Versatile peroxidase (VP, EC 1.11.1.16) constitutes the third family of ligninolytic peroxidases, which was described 20-years ago. VP combines catalytic properties of the above two families due to the presence of both a Mn-oxidation site and a catalytic tryptophan in its molecular structure. In the present work, VP (isoenzyme VPL2) from Pleurotus eryngii has been subjected to protein engineering using a rational design strategy.

A high number of basic residues with their side chains exposed to the solvent, most of them with no movement restrictions by interactions with surrounding amino acids, were identified in MnP4 (31 of a total of 34 present in the protein, including 20 lysines and 11 arginines). Seven of these exposed residues (4 lysines and 3 arginines) were introduced into VPi, and the VPi-br variant containing the 8 mutations present in VPi plus mutations T2K/A131K/Q219K/L288R/A308R/A309R/A314R was obtained. The analysis of the VPi-br crystal structure also revealed that the seven solvent-exposed basic residues introduced in this variant present a configuration similar to that observed for the homologous residues in MnP4. Their side-chains appear interacting with water molecules through hydrogen bonds or do not present any interaction, and no contacts are observed with surrounding residues. VPi-br and VPi-ss crystal structures exhibited minor differences compared with VPi regarding the interactions involving the mutated residues in region A (VPi-br also regarding the interactions of residues in region C), and no significant changes were identified in the other regions described. VPi-br harboring seven additional basic residues exposed to the solvent, and VPi-ss containing two cysteines added to form an additional extra disulfide bond, further improved the stability of VPi at acidic pH (respectively). Both variants retained 86% and 85% of the initial activity at pH 3.5 after 24 h of incubation compared to the 61% retained by VPi and far from the 1% of the native VP. In our case, the increased stability of VPi-br at acidic pH compared with VPi could be explained by a general stabilizing effect of the extra basic residues participating in charge-charge interactions with other charged amino acids of the protein surface (although these interactions were not observed in the VPi-br crystal structure) and by interacting with the solvent improving the solubility of the protein. It should be also noted that the polar surface of the VPi-br variant is significantly increased with respect to VPi by replacing five hydrophobic residues (four alanines and leucine) with polar charged amino acids (four arginines and one lysine). Unlike what observed at low pH, VPi-ss only exhibited a slight increased stability after 1 h incubation at pH 7 compared with VPi. Both VPi-br and VPi-ss not only did not show an additional improvement at longer times at neutral pH but, on the contrary, VPi-br significantly reversed the improvement attained in VPi.

> AKCDDGRTTANAACCILFPILDDIQENLFDGAQCGEEVHESLRLTFHDAIGFSPTLGGGGADGSIIAFSDIETNFPANAGIDEIVEAQKPFVAKHNISAGDFIQFAGAVGVSNCPGGVRIPFFLGRPDAVKASPDHLVPEPFDSVTSILARMGDAGFSPVEVVWLLASHSIAAADKVDPSIPGTPFDSTPGVFDSQFFIETLLKGRLFPGTADNKGEAKSPLQGEIRLQSDELLARDPRTACEWQSMVNNQPKIQNRFAATMSKMALLGQDKTKLIDCSDVIPTPPARVGAAHLPAGFSLKDVEQACRKTPFPRLTADPGPVTSVPPVPGS> AIKKDQKAPIITIFDNRGCEVKKNNYSGAKANGMEDDQCVKLTMETITVSETTAAKKLQEFIGLKAT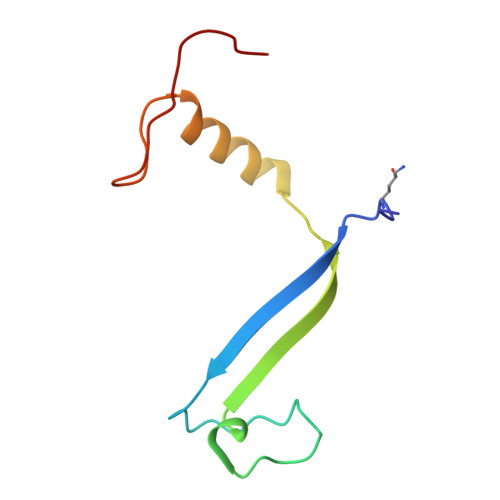AINVPQISGVTKKY>MHHHHHHGSNINKAKVASVESDYSSVKSAALSYYSDTNK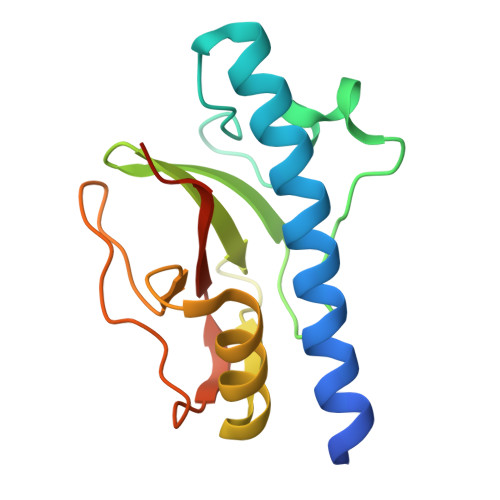IPVTPDGQTGLSVLETYMESLPDKADIGGKYKLIKVGNKLVLQIGTNDEGVTLTEAQSAKLLSDIGENKIYTSVTADNLGNPLTSNTKVDNKVLYIVLIDNTVMDSTK[3x]Recently, the novel multifunctional S-adenosyl-1-methionine (SAM)-dependent enzyme LepI, located in the PKS-NRPS gene cluster for leporin biosynthesis, was characterized in Aspergillus flavus. LepI is considered as a SAM-dependent methyltransferase that can catalyze stereoselective dehydration via three pericyclic transformational processes: intramolecular Diels-Alder and hetero-Diels-Alder reactions and a retro-Claisen rearrangement. The overall structure was found to be largely similar to that of SAM-dependent enzymes,28–31 exhibiting a core α/β fold of alternating β strands (β1–β7) and α helices (α1–α19). This structure exhibiting α helices and β sheets comprises an all-helix amino-terminal domain (NTD), a carboxy-terminal domain including a substrate-binding site, and a SAM-binding site, which is formed by a seven-stranded β sheet rounded with five helices.

To elucidate the mechanism of LepI action, we first determined the structure of SAM/MTA-bound LepI at a high resolution of 1.7 Å. Two molecules of LepI observed in an asymmetric crystal unit form the homodimer, which is primarily mediated by the NTD; specifically, the α1 and α2 segments of one subunit interact with those of another subunit to form interlocking fingers, and α3 is involved in the formation of the hind surface of the active site. As determined from the strong electron density, SAM binds to one side of the LepI pocket and maintains the catalytic domain in the active state through interaction networks. The adenosine rings and amino acids of SAM interact with Phe276 and Asn275 via π–π interaction and salt bonding, respectively. O4 of the ribose and the tail amide of SAM form a pair of hydrogen bonds with the main chain of Gly227. Specifically, a hydrogen bond forms between the S+-CH3 moiety and the main chain of Leu292. Collectively, these interactions result in the coordination of SAM in an extended confirmation. Additional electron density was observed in the pocket of the LepI density map, located opposite the SAM-binding site. As MTA could be detected via HPLC analysis of the purified proteins compared with the reference standard of SAM and MTA, we modeled MTA in the electron-dense cluster and found it likely to be coordinated in the hydrophobic site, with some residues displaying significant conformational changes upon MTA binding. MTA probably mimics the substrate binding at the active site, thereby blocking the entry of a native substrate as a competitive inhibitor, thereby decreasing LepI activity.

>[2x]METVAAIKTLIQQLAQSTDQFGRAEINDALRELQYSLETPFDTVMRMSLDTCQVAVARIGSDLGLFKHLSQCASPQSAEELADHLGCGRELMSRLLRYMASVRMVQQTDDIKYISSNITQTLAVPGLEAGMRHAFENLWPVLMALPDFLAERKYPDIVDAKDTAFQKAFNTDQDCFHWLATQPTRIANFKVLLTDERTPNFLSTFPLEKELGSWSAEPEKALFVDIGGGMGHACIRLREKYPNQPGRVILQDLPPVLQAAQATLPLSGIESMPHNFHTPQPVQGAKFYFLRLILRDFPDHQALEILQNIVPAMDAESRIVIDDGVPPEKGARWAETGTDICIMSALGSKERTQRQWEELAAKAGLQLQALYQYTWPVVNAAMVFSLQ>GPLGSAAASFGQTKIPRGNGPYSVGCTDLMFDHTNKGTFLRLYYPSQDNDRLDTLWIPNKEYFWGLSKFLGTHWLMGNILRLLFGSMTTPANWNSPLRPGEKYPLVVFSHGLGAFRTLYSAIGIDLASHGFIVAAVEHRDRSASATYYFKDQSAAEIGDKSWLYLRTLKQEEETHIRNEQVRQRAKECSQALSLILDIDHGKPVKNALDLKFDMEQLKDSIDREKIAVIGHSFGGATVIQTLSEDQRFRCGIALDAWMFPLGDEVYSRIPQPLFFINSEYFQYPANIIKMKKCYSPDKERKMITIRGSVHQNFADFTFATGKIIGHMLKLKG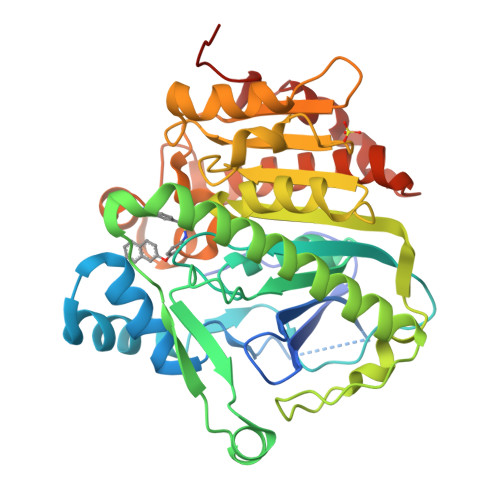DIDSNVAIDLSNKASLAFLQKHLGLHKDFDQWDCLIEGDDENLIPGTNINTTNQHI[2x]N-(cyclobutylmethyl)-3-{5-[1-(pyrrolidin-1-yl)cyclohexyl]-2-(1-{[(2S)-pyrrolidin-2-yl]methyl}-1H-indol-5-yl)-1,3-thiazol-4-yl}prop-2-yn-1-amine 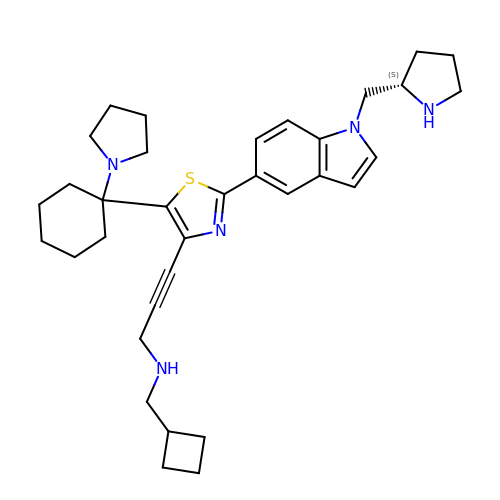| C34 H45 N5 S | FHCOGWJRKLTMNQ-LJAQVGFWSA-N> MEPSSLELPADTVQRIAAELKCHPTDERVALHLDEEDKLRHFRECFYIPKIQDLPPVDLSLVNKDENAIYFLGNSLGLQPKMVKTYLEEELDKWAKIAAYGHEVGKRPWIT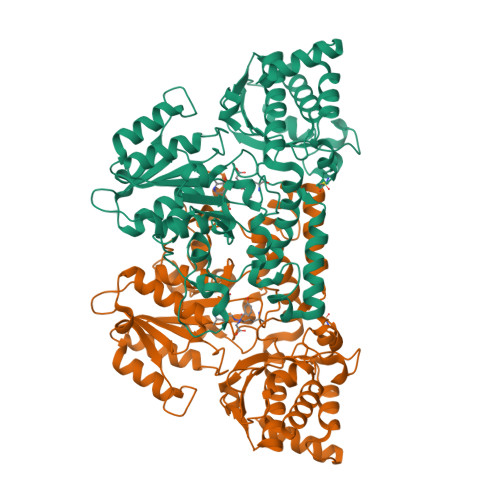GDESIVGLMKDIVGANEKEIALMNALTVNLHLLMLSFFKPTPKRYKILLEAKAFPSDHYAIESQLQLHGLNIEESMRMIKPREGEETLRIEDILEVIEKEGDSIAVILFSGVHFYTGQHFNIPAITKAGQAKGCYVGFDLAHAVGNVELYLHDWGVDFACWCSYKYLNAGAGGIAGAFIHEKHAHTIKPALVGWFGHELSTRFKMDNKLQLIPGVCGFRISNPPILLVCSLHASLEIFKQATMKALRKKSVLLTGYLEYLIKHNYGKDKAATKKPVVNIITPSHVEERGCQLTITFSVPNKDVFQELEKRGVVCDKRNPNGIRVAPVPLYNSFHDVYKFTNLLTSILDSAETKN> SNAMTEEHVVLLDEQDKPSGTLEKYAAHTLNTPLHLAFSCWLFNEDGQLLVTRRSLSKKAWPGVWTNSVCGHPQQGETTEEAIIRRCRFELGVEITDLTPV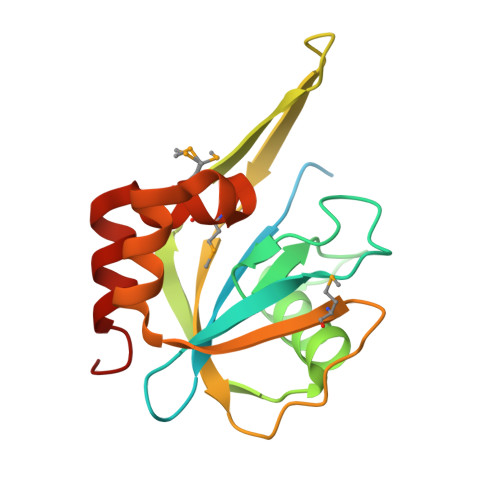YPHFSYRATDPNGIVENEVCPVFAARATSVLQVNSEEVMDYQWSEFKSVWKSLLATPWAFSPWMVMQASDEQARERLLNYCQR>[2x]MKMTFFPYELKLRHVFTVATYSRTTTPDVQVEIEYEGVTGYGEASMPPYLGETVESVMNFLKKVNLEQFSDPFQLEDILSYVDSLSPKDTAAKAAVDIALHDLVGKLLGA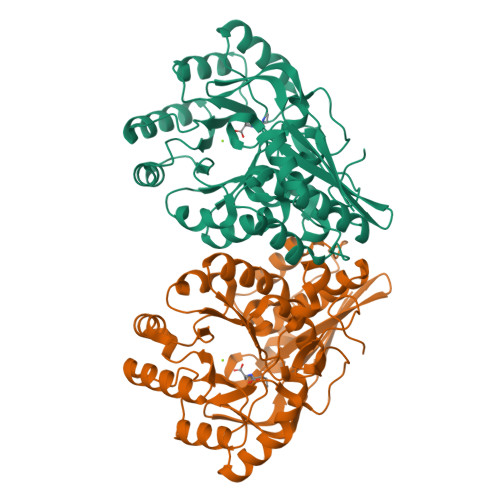PWYKIWGLNKEKTPSTTFTIGIDTPDVVRAKTKECAGLFNILKVKLGRDNDKEMIETIRSVTDLPIAVDANQGWKDRQYALDMIHWLKEKGIVMIEQPMPKEQLDDIAWVTQQSPLPVFADESLQRLGDVAALKGAFTGINIKLMKCTGMREAWKMVTLAHALGMRVMVGCMTETSCAISAASQFSPAVDFADLDGNLLISNDRFKGVEVVNGKITLNDLPGIGVMKI> MRALLPYLALYKRHKWMLSLGIVLAIVTLLASIGLLTLSGWFLSASAVAGVAGLYS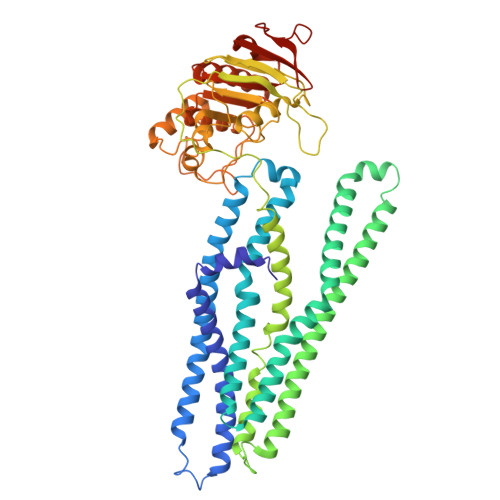FNYMLPAAGVRGAAITRTAGRYFERLVSHDATFRVLQHLRIYTFSKLLPLSPAGLARYRQGELLNRVVADVDTLDHLYLRVISPLVGAFVVIMVVTIGLSFLDFTLAFTLGGIMLLTLFLMPPLFYRAGKSTGQNLTHLRGQYRQQLTAWLQGQAELTIFGASDRYRTQLENTEIQWLEAQRRQSELTALSQAIMLLIGALAVILMLWMASGGVGGNAQPGALIALFVFCALAAFEALAPVTGAFQHLGQVIASAVRISDLTDQKPEVTFPDTQTRVADRVSLTLRDVQFTYPEQSQQALKGISLQVNAGEHIAILGRTGCGKSTLLQQLTRAWDPQQGEILLNDSPIASLNEAALRQTISVVPQRVHLFSATLRDNLLLASPGSSDEALSEILRRVGLEKLLEDAGLNSWLGEGGRQLSGGELRRLAIARALLHDAPLVLLDQPTEGLDATTESQILELLAEMMREKTVLMVTHRLRGLSRFQQIIVMDNGQIIEQGTHAELLARQGRYYQFKQGL> G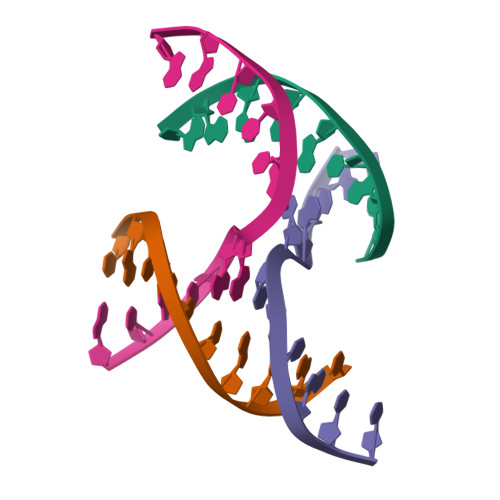GATGCACA;> CACACCGTAC;> TGTGCTGTGCT;> GTACGGATCCAG> MGKNLSLRQDDAQHALSANTSSAYNSVYDFLRYHDRGDGLTVNGKTSYSIDQAAAQITRENVSWNGTNVFGKSANLTFKFLQSVSSIPSGDTGFVKFNAEQIEQAKLSLQSWSDVANLTFTEVTGNKSANITFGNYTRDASGNLDYGTQAYAYYPGNYQGAGSSWYNYNQSNIRNPGSEEYGRQTFTHAIGHALGLAHPGEYNAGEGDPSYNDAVYAEDSYQFSI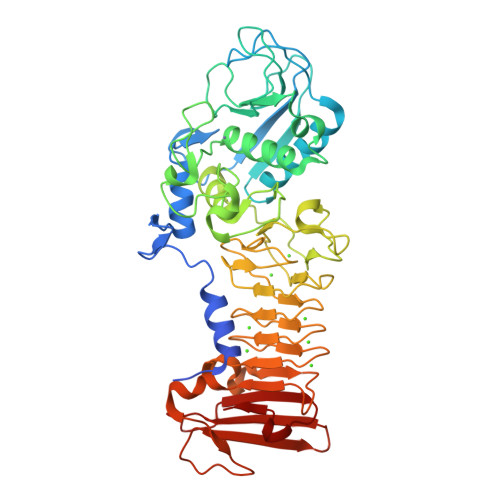MSYWGENETGADYNGHYGGAPMIDDIAAIQRLYGANMTTRTGDSVYGFNSNTDRDFYTATDSSKALIFSVWDAGGTDTFDFSGYSNNQRINLNEGSFSDVGGLKGNVSIAHGVTIENAIGGSGNDILVGNSADNILQGGAGNDVLYGGAGADTLYGGAGRDTFVYGSGQDSTVAAYDWIADFQKGIDKIDLSAFRNEGQLSFVQDQFTGKGQEVMLQWDAANSITNLWLHEAGHSSVDFLVRIVGQAAQSDIIV>[2x]MSKIERISAFLNDKEVDMTFITNPTTLNYLTGLAIDPSERIAGLMIFRDSTPMLFTPALEVEKAKEHTSGLDIFGYEDSQNPWEVVKNHVKSDVKSIAVEFSDIPLAKTEGLKAQFGDINFVNLTPLIERMRLIKSADEIEKMKVAGDFADKCFEIGFATAAERN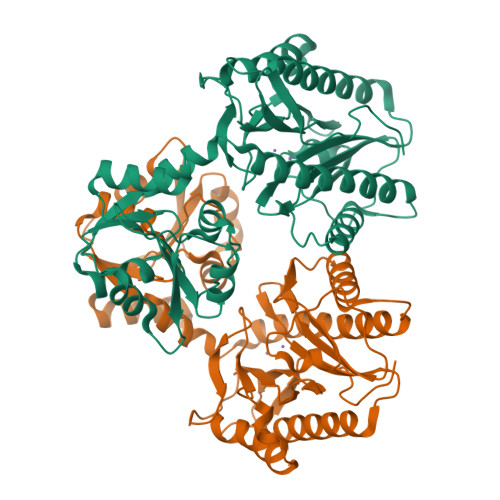GVTESDIVAKIEYEMKRMGVPQMSFDTLVLSGARAANPHGAPENVEIQENKLLLFDLGVMSGGYASDATRTIAIGQPNDFDAEIHKIVKEAQQAAMDFIKPGVTAHEVDAVARDLITKAGYGEYFNHRLGHGIGMDVHEYPSIVAGNDLVIQEGMCFSNEPGIYIPGKVGVRIEDCLYVTENGCESFTHTDHDLLIF> MPPKAKAKDAGPVERPILGRFSSHLKIGIVGLPNVGKSTLFNTLTKLSIPAENFPFCTIEPNEARVNIPDERFDWLCQTYKPKSEIPAFLEIHDIAGLVRGAHEGQGLGNNFLSHIRAVDGIFHVLRAFEDADIIHVDDIVDPVRDLETITEELRLKDIEFVGKKIDDVEKSMKRSNDKQLKIELELLQKVKAWLEDGKDVRFGDWKTADIEILNTFQLLSAKPVVYLINLNERDYQRKKNKFLPKIHAWVQEHGGDTMIPFSGVFERSLADMAPDEAAKYCEENKLQSALPRIIKTGFSAINLIYFFTAGPDEVKCWQIRRQSKAPQAAGAIHTDFERGFICAEVMKFEDLKELGNEPAVKAAGKYRQEGKTYVVQDGDIIFFKFNVSGGGKK

AtYchF1 is an unconventional G-protein in Arabidopsis thaliana that exhibits relaxed nucleotide-binding specificity. AtYchF1 in Arabidopsis thaliana is a close homolog of OsYchF1, which possesses a noncanonical G4 sequence (NxxE) within the G domain, instead of the canonical NKxD in most P-loop GTPases, resulting in a relaxed nucleotide-binding specificity and the ability to hydrolyze both ATP and GTP. Similar to OsYchF1, AtYchF1 was also previously characterized as negative regulator for both biotic and abiotic stresses. OsYchF1 harbors a G domain at the N-terminus for GTP and ATP binding and hydrolysis, and a TGS (ThrRS, GTPase, and SpoT) domain in the C-terminus for nucleic acid binding.

The structure of AtYchF1-ppGpp with Mg2+ was resolved using X-ray crystallography at 2.07Å. In the structure of the AtYchF1-ppGpp complex, the ppGpp molecule was bound at the normal nucleotide-binding site of the G domain, as expected. The guanine moiety of ppGpp was engaged in π-stacking interactions with the Loop A motif, sandwiched between the hydrophobic chains of Phe129 and Val265 (corresponding to Ala265 in OsYchF1). The O6 of the guanine ring was recognized by the well-described side-chain of Asn230 of the G4 element. The α- and β-phosphates of ppGpp were coordinated by the G1 motif (P-loop), and an Mg2+ was coordinated by the β-phosphate and the side-chain of Ser38 in the G1 motif. The δ- and ε-phosphates, which were covalently bound to the 3′-OH group of the ribose moiety, discriminated ppGpp from its GDP counterpart by pointing away from the active site. A salt bridge between the δ-phosphate and Arg268 was observed. The binding of ppGpp had a greater stabilizing effect on the conformation of Loop A (Arg127-Asp142), with His136 as the most significantly stabilized. However, in the AtYchF1-ppGpp structure, His136 was stabilized by Asp131 which had a hydrophilic interaction with the guanine moiety of ppGpp. Interestingly, the distance between the TGS and helical domains of the AtYchF1-ppGpp complex is 4.7 Å shorter than those in the OsYchF1-AMPPNP or OsYchF1-GMPPNP complex.>[4x]KIQVKCSAPNSVTITNASGGLYLVEYPEGYVAYSKATEVTGKLVHANFGTKKDFEDLDYAVNGSIVIVRAGKITIAEKVANAQSFNAIGVLIYKDRTKYPISRADEPLQGHSG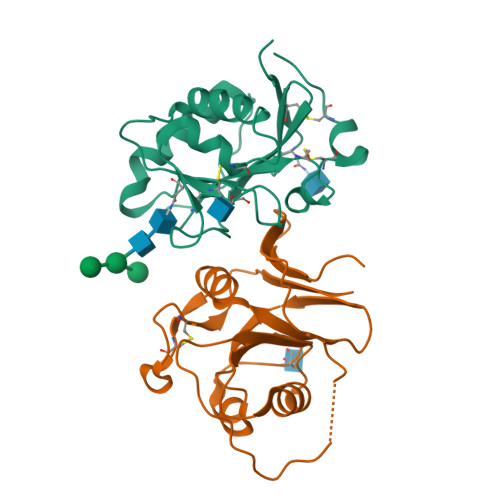LPSIPVQTISREAAEKLFQNMERDCPRSWNTDSSCKLELLQNRNVKLTVNNCLKEGTSGHHHHHH;>[4x]SNELPSLCMLNNSFYYMRGGVNTFLIRVSDISVLMKEYDVSIYEPEDLGNCLNKSDSSWAIHWFSNALGHDWLMDPPMLCRNKTKKEGSNIQFNISKADDARVYGKKIRNGMRHLFRGFHDPCEEGKVCYLTINQCGDPSSFDYCGVNHLSKCQFDHVNTGSHHHHHH>[4x]MTSVQLETPHSGKYEQPTGLFINNEFVKGQEGKTFDVINPSDESVITQVHEATEKDVDIAVAAARKAFEGSWRQ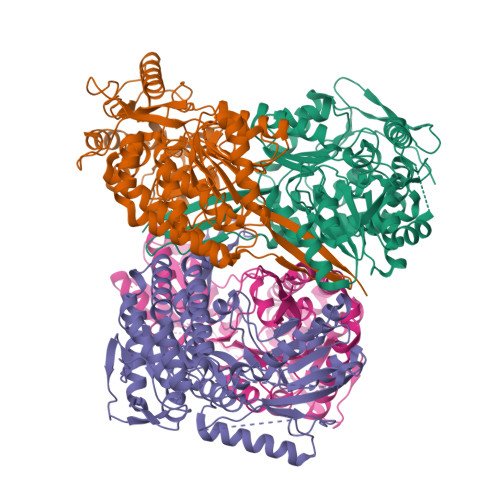ETPENRGKLLNNLANLFEKNIDLLAAVESLDNGKAISMAKGDISMCVGCLRYYGGWADKITGKVIDTTPDTFNYVKKEPIGVCGQIIPWNFPLLMWAWKIGPAIACGNTVVLKTAEQTPLGGLVAASLVKEAGFPPGVINVISGFGKVAGAALSSHMDVDKVAFTGSTVVGRTILKAAASSNLKKVTLELGGKSPNIVFEDADIDNAISWVNFGIFFNHGQCCCAGSRVYVQESIYDKFVQKFKERAQKNVVGDPFAADTFQGPQVSKVQFDRIMEYIQAGKDAGATVETGGKRKGDKGYFIEPTIFSNVTEDMKIVKEEIFGPVCSIAKFKTKEDAIKLGNASTYGLAAAVHTKNLNTAIEVSNALKAGTVWVNTYNTLHHQMPFGGYKESGIGRELGEDALANYTQTKTVSIRLGDALFG> GAKNYYDITLALAGICQSARLVQQLAHQGHCDADALHVSLNSIIDMNPSSTLAVFGGSEANLRVGLETLLGVLNASSRQGLNAELTRYTLSLMVLERKLSSAKGALDTLG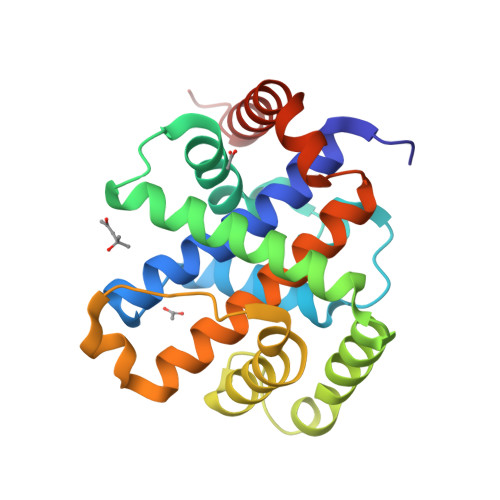NRINGLQRQLEHFDLQSETLMSAMAAIYVDVISPLGPRIQVTGSPAVLQSPQVQAKVRATLLAGIRAAVLWHQVGGGRLQLMFSRNRLTTQAKQILAHLTPEL> MRNKIFISHATPDDNDFTRWLALKLIGLGYEVWCDILFLDKGVDFWSNIEKVIREDTCKFLLVSSSYSNQREGVLKELAVAAKVKKQLKDDKFIIPLAIDEQLSYDDINIDIVRLNAIDFKMSWARGLKDILEAFEKQKVPKEVADASKSNLLYQQIFLHDKSVIEKEEIYDSNWLSILSFPEELRFHEYNWMLPKRFDVRELTFPAVRYKNYLCTFAWAYDFTYHLPKTETYHKSKTIRIPTEEILSGSYDSNFIRNAECKRLIVQLLNKAFELRMKDKEVQEYEMSNK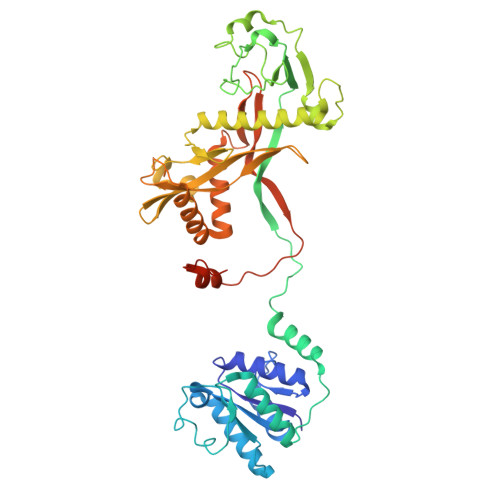TAYWLEKGKLEKDKFEKTMLVGKQKDKNWHFAISGASKLYPFPVLMISSHIFFTADGKKLIDSSSVQHSSRRRQGKNWWNNTWRTKLLAFIKYLSDDDTSFYLEMGSEEKVFVSNEPVKFKGNVSYNIPEKNTLEEEAELSGFNQGEDIEELEELIENLEAE>[2x]GSHNMAEMVETVCGPVPVEQLGKTLIHEHFLFGYPGFQGDVTRGTFREDESLRVAVEAAEKMKRHGIQTVVDPTPNDCGRNPAFLRRVAEETGLNIICATGYYYNGEGAPPYFQ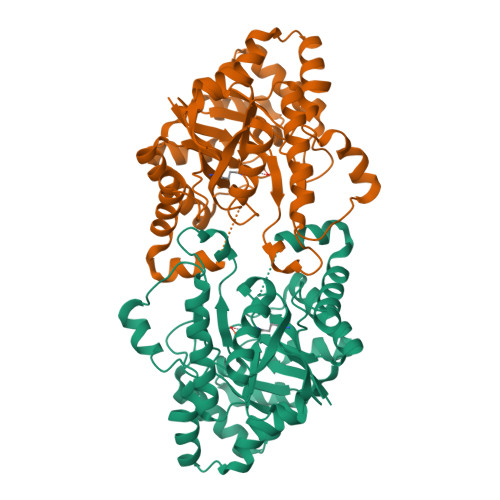FRRLLGTAEDDIYDMFMAELTEGIADTGIKAGVIKLASSKGRITEYEKMFFRAAARAQKETGAVIITHTQEGTMGPEQAAYLLEHGADPKKIVIGHMCGNTDPDYHRKTLAYGVYIAFDRFGIQGMVGAPTDEERVRTLLALLRDGYEKQIMLSHDTVNVWLGRPFTLPEPFAEMMKNWHVEHLFVNIIPALKNEGIRDEVLEQMFIGNPAALFSA> GPMDRYQRKIGCFIQIPNLGRGQLKYVGPVDTKAGMFAGVDLLANIGKNDGSFMGKKYFQTEYPQSG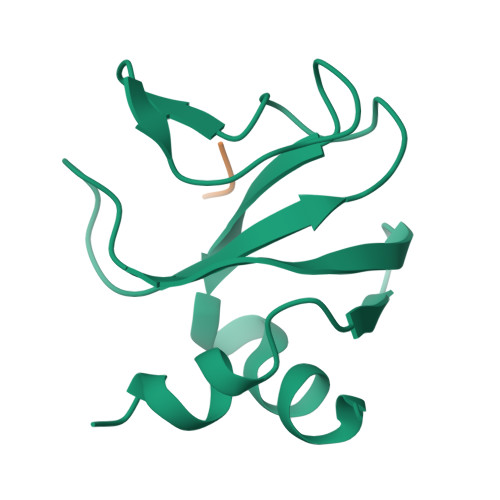LFIQLQKVASLIEKASISQTSRRTTMEPLSIPKNR;> SNNLIIDEETF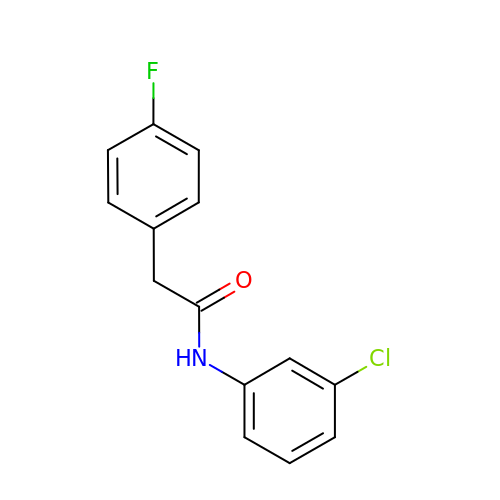N-(3-chlorophenyl)-2-(4-fluorophenyl)acetamide | C14 H11 Cl F N O | BNRVDRRNZNBFGG-UHFFFAOYSA-N>ARKCSLTGKWTNDLGSNMTIGAVNSRGEFTGTYITAVTATSNEIKESPLHGTQNTINKRTQPTFGFTVNWKFSES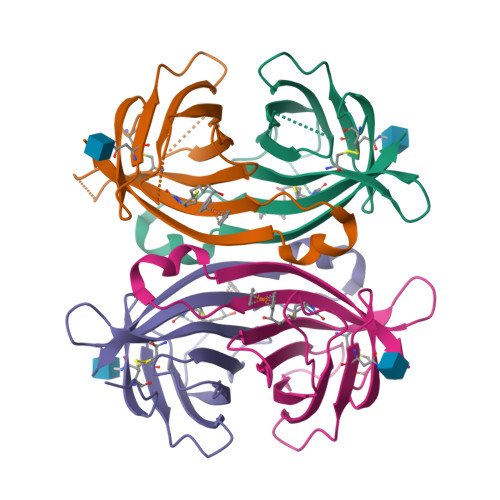TTVFTGQCFIDRNGKEVLKTMWLLRSSVNDIGDDWKATRVGINIFTRLRTQKE[4x]> MLRRSDLLLKKGWTHNPGRTRRGGKNLAWRPKMSERTLEQFVPLHLAFPRRHPNSWQERQFHLLGYVKWPKEIGFYNAGDNFELTPQAAYRIYKQNCDETFWTRLHNEKTIIHLLP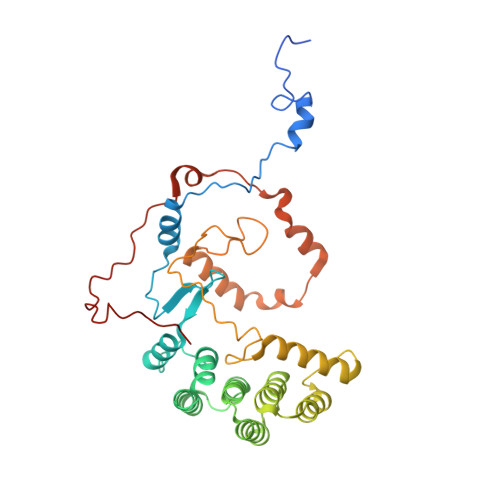LVEQDPGTNMVLVDDIFRHHLKRFGADHYIYNAVMQAAAFAKDFPRCEQLLAEMRGLGLEPNAQSYVNMMLGARLTGKPRDQAEAFFREGIKTGAISAVMRLDTEFQMWMNQLERLGSFKAKVGYLSVNEEGASPMPRDMWALWGWHRTEAKFISRKQMISEQVQNRVRSGKELVGTVYQKARRQPWAKYNGMFPYDYNGPARRPAASFVDAPTPTHNAEVCGTAY>[2x]ADPKCTVSHEVADCSHLKLTQVPDDLPTNITVLNLTHNQLRRLPAANFTRYSQLTSLDVGFNTISKLEPELCQKLPMLKVLNLQHNELSQLSDKTFAFCTNLTELHLMSNSIQKIKNNPFVKQKNLITLDLSHNGLSSTKLGTQVQLENLQELLLSNNKIQALKSEELDIFANSSLKKLELSSNQIKEFSPGCFHAIGRLFGLFLNNVQLGPSLTEKLCLELANTSIRNLSLSNSQLSTTSNTTFLGLKWTNLTMLDLSYNNLNVVGNDSFAWLPQLEYFFLEYNNIQHLFSHSLHGLFNVRYLNLKRSFTKQSISLASLPKIDDFSFQWLKCLEHLNMEDNDIPGIKSNMFTGLINLKYLSLSNSFTSLRTLTNETFVSLAHSPLHILNLTKNKISKIESDAFS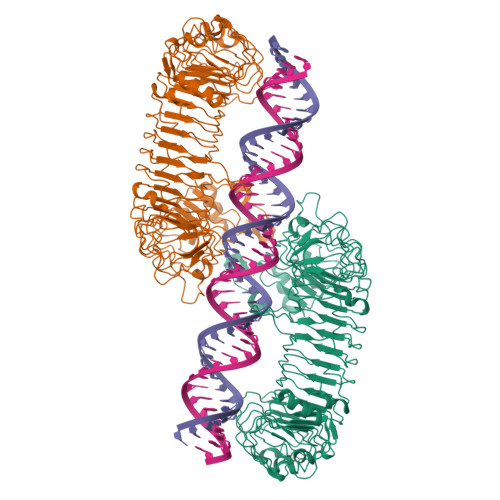WLGHLEVLDLGLNEIGQELTGQEWRGLENIFEIYLSYNKYLQLTRNSFALVPSLQRLMLRRVALKNVDSSPSPFQPLRNLTILDLSNNNIANINKKMLKGLEKLEILDLQHNNLARLWKHANPGGPIYFLKGLSHLHILNLESNGFDEIPVEVFKDLFELKIIDLGLNNLNTLPASVFNNQVSLKSLNLQKNLITSVEKKVFGPAFRNLTELDMRFNPFDCTCESIAWFVNWINETHTNIPELSSHYLCNTPPHYHGFPVRLFDTSSCKHHHHHH Chlorite dismutases (Clds) are heme b-containing oxidoreductases that can decompose chlorite to chloride and molecular oxygen. The two clades exhibit differences in (i) oligomerization, with clade 1 proteins being homopenta- or homohexamers6−10 and clade 2 representatives forming homodimers,11−14 and (ii) subunit structure, with “long” clade 1 Clds being composed of an N-terminal and a C-terminal heme b-carrying ferredoxin-like domain and “short” clade 2 proteins lacking the α-helices of the N-terminal domain. The only charged amino acid in the hydrophobic distal heme cavity is a fully conserved arginine (R173 in NdCld and R127 in CCld), which is proposed to be flexible and to switch between two conformations during catalysis, i.e., pointing toward either the heme iron (“in”) or the substrate entry channel (“out”).4,6,8,11,14,16 Importantly, the hydrogen-bonding network of this catalytic arginine is different in clade 1 and clade 2 Clds. In clade 2 Clds, R127 is H-bonded to Q74 located on a flexible α-helical loop, which in general connects the N-terminal and C-terminal ferredoxin-like domains in porphyrin-binding α + β barrel proteins.

As typical for a clade 2 Cld, its distal arginine 127 is hydrogen-bonded to glutamine 74. The latter has been exchanged with either glutamate (Q74E) to arrest R127 in a salt bridge or valine (Q74V) that mirrors the setting in clade 1 Clds. The Q74V variant mirrors the situation in the clade 1 representative NdCld and should exhibit an increased flexibility of R127 compared to that of wild-type CCld, whereas Q74E might arrest the catalytic amino acid by forming a salt bridge. We provide the crystal structures of Q74V and Q74E and demonstrate the impact of the mutations and pH on heme coordination and active site architecture by ultraviolet–visible (UV–vis), electron paramagnetic resonance (EPR), and electronic circular dichroism (ECD) spectroscopy. Besides heme coordination, the mutations are shown to have a strong impact on the thermal stability of the heme cavity but an only weak effect on the chlorite degradation activity. The conformational dynamics of R127 is shown to have a significant role in heme coordination during the alkaline transition and in the thermal stability of the heme cavity, whereas its impact on the catalytic efficiency of chlorite degradation is relatively small.

>[2x]GPGYQDPNNRYSFIGGRTGQWQVVKIRNVLGPGLQLVEKVNILNGAVAEIPLDSAWRLQGFASNIRYAIRTELEALQAVEPMLNRAEAILAVLIPIKKSAQWWEMAQDERRDIFERESHHTAVGLEYLPGVARRLLHCRDLGEEFDFLTWFEFAPEHSSAFNELLLRMRASKEWEYVEREVEVWLKRL> RSTDTFNYATYHTLEEIYDFLDLLVAENPHLVSKIQIGNTYEGRPIYVLKFSTGGSKRPAIWIDTGIHSREWVTQASGVWFAKKITQDYGQDAAFTAILDTLDIFLEIVTNPDGFAFTHSTNRMWRKTRSHTAGSLCIGVDPNRNWDAGFGLSGASSNPCSETYHGKFANSEVEVKSIVDFVKDHGNIKAFISIHSYSQL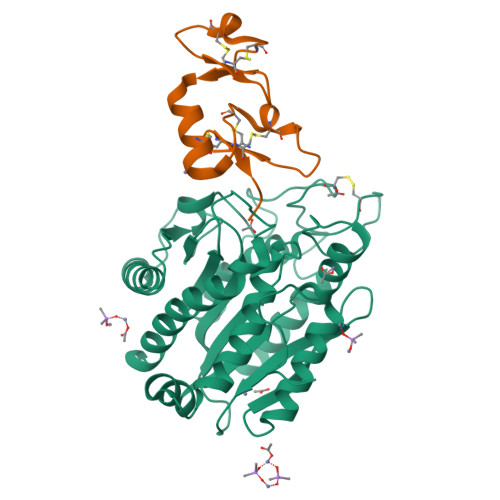LMYPYGYKTEPVPDQDELDQLSKAAVTALASLYGTKFNYGSIIKAIYQASGSTIDWTYSQGIKYSFTFELRDTGRYGFLLPASQIIPTAKETWLALLTIMEHTLNHP;> VRKCLSDTDCTNGEKCVQKNKICSTIVEIQRCEKEHFTIPCKSNNDCQVWAHEKICNKGCCWDLL>[2x]MAHHHHHHVDDDDKMAGDSAAYQRTSLYGDDVVIVAAHRTPLCKSKRGNFKDTYPDDLLAPVLRALIEKTNLNPSEVGDIVVGTVLAPGSQ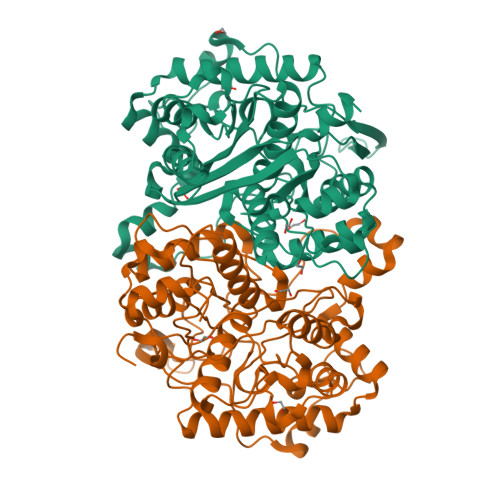RASECRMAAFYAGFPETVAVRTVNRQCSSGLQAVADVAAAIKAGFYDIGIGAGLESMTTNPMAWEGSVNPAVKKFAQAQNCLLPMGVTSENVAQRFGVSRQEQDQAAVDSHRKAAAATAAGKFKDEIIPVKTKLVDPKTGDEKPITVSVDDGIRPTTTLASLGKLKPVFKKDGTTTAGNSSQVSDGAGAVLLMKRSVAMQKGLPVLGVFRTFAAVGVDPAIMGIGPAVAIPAAVKAAGLELDDIDLFEINEAFASQFVYCRNKLGLDPEKINVNGGAMAIGHPLGATGARCVATLLHEMKRRGKDCRFGVVSMCIGTGMGAAAVFERGDGVDELRNARKVEAQGLLSKDAR> GEDVFEVEKILDMKTEGGKVLYKVRWKGYTSDDDTWEPEIHLEDCKEVLLEFRKKIAENKAK;> YEPSTTARKVGRP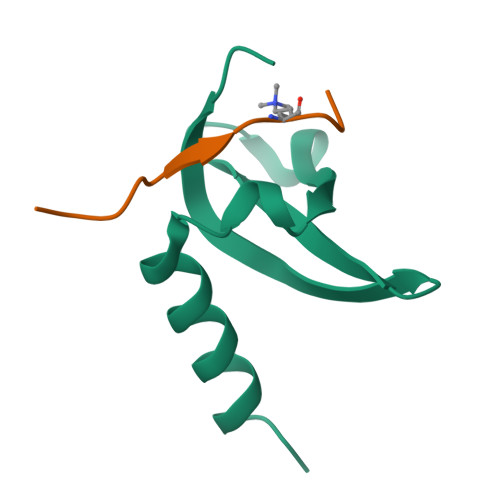GR>GGCUAGCUGGAGGGGCGCCAGUUCGCUGGUGGUUGGGUGCGGUCGGCUAGCC[2x]

The Chili RNA aptamer mimics large Stokes shift fluorescent proteins and exhibits high affinity for 3,5-dimethoxy-4-hydroxybenzylidene imidazolone (DMHBI) derivatives to elicit green or red fluorescence emission. The Chili RNA folds into a single coaxial helical stack with a length of ~70 Å that contains two A-form duplexes P1 and P2 that are separated by the central fluorophore binding domain (FBD). The P1 stem transitions via a base triple into a two-tiered G-quadruplex, which constitutes the core of the FBD. The ligand is immobilized by π-stacking between an unusual G14:G31 base pair and the T2 quartet.

The 52-nt Chili RNA aptamer was co-crystallized with two of its cognate ligands, DMHBO+ and DMHBI+. Crystals were derivatized with iridium(III) hexammine (by soaking or co-crystallization), experimental phases were obtained by single-wavelength anomalous dispersion (SAD), and the initial models were used for molecular replacement (MR) with native datasets.>[4x]GAMGSSSVWGVAFSPDGQTIASASDDKTVKLWNRNGQLLQTLTGHSSSVWGVAFSPDGQTIASA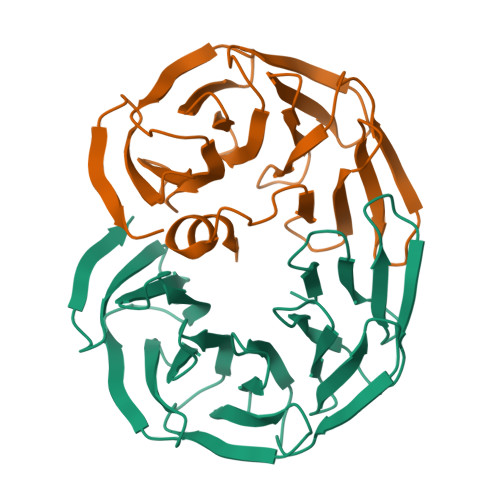SDDKTVKLWNRNGQLLQTLTGHSSSVWGVAFSPDGQTIASASDDKTVKLWNRNGQLLQTLTGHSSSVWGVAFSPDGQTIASASDDKTVKLWNRNGQLLQTLTGHSSSVWGVAFSPDGQTIASASDDKTVKLWNRNGQLLQTLTGH BoNTs are synthesized as a single polypeptide chain (150 kDa), which is post-translationally cleaved into a di-chain molecule composed of light chain (LC, 50 kDa) and heavy chain (HC, 100 kDa). LC is the catalytic domain and a zinc-endopeptidase, while HC is further divided into two sub-domains of equal molecular mass called the translocation domain (Hn) and the membrane binding domain (Hc). Inhibition of neurotransmission takes place by proteolysis of one of the SNARE proteins that mediate cell secretion. Synaptobrevin (or VAMP) was identified as the BoNT/D specific substrate and is cleaved at the Lys59-Leu60 position.

The crystal of LHn/D diffracted at 2.3 Å resolution in space group P6422 with cell dimensions a = b = 173, c = 222 Å; α = β = 90, γ = 120°. Despite the large unit cell, a single molecule was present in the asymmetric unit corresponding to an unusually high solvent content of 75%. The X-ray crystal structure presents the two domains, LC and Hn, in a close interaction. No electron density was observed for regions 442–457 (between the two domains), residues 494–510, and the C-terminal poly-histidine tag (last fifteen residues), all in solvent-accessible areas. Additionally, one of the most intriguing features of BoNT, the ‘belt’ region (residues 458–547), which is part of Hn and surrounds LC, was visible in the electron density map (despite high solvent content in the crystal) in the structure presented here and highlights the intricate interactions between the two domains. A PISA22 analysis shows that the LC-belt interaction is supported by over 40 potential hydrogen bonds and 2 salt bridges, making up a 3373 Å2 contact area. Loss of the zinc ion was confirmed with a local rearrangement of the active site residues. Mutation of the zinc-coordinating H233 to tyrosine caused displacement of the catalytic ion, replaced in its position with the Y233 hydroxyl group. Overall, the role of the zinc ion appears mostly catalytic with little impact on the structural integrity of the light chain.

> MTWPVKDFNYSDPVNDNDILYLRIPQNKLITTPVKAFMITQNIWVIPERFSSDTNPSLSKPPRPTSKYQSYYDPSYLSTDEQKDTFLKGIIKLFKRINERDIGKKLINYLVVGSPFMGDSSTPEDTFDFTRHTTNIAVEKFENGSWKVTNIITPSVLIFGPLPNILDYTASLTLQGQQSNPSFEGFGTLSILKVAPEFLLTFSDVTSNQSSAVLGKSIFCMDPVIALMHQLTYSLHQLYGINIPSDKRIRPQVSEGFFSQDGPNVQFEELYTFGGLDVEIIPQIERSQLREKALGHYKDIAKRLNNINKTIPSSWISNIDKYKKIFSEKYNFDKDNTGNFVVNIDKFNSLYSDLTNVMSEVVYSSQYNVKNRTHYFSRHYLPVFANILDDNIYTIRDGFNLTNKGFNIENSGQNIERNPALQKLSSESVVDLFTKVCVDKSEEKLYDDDDKDRWGSSLQCIKVKNNRLPYVADKDSISQEIFENKIITDETNVQNYSDKFSLDESILDGQVPINPEIVDPLLPNVNMEPLNLPGEEIVFYDDITKYVDYLNSYYYLESQKLSNNVENITLTTSVEEALGYSNKIYTFLPSLAEKVNKGVQAGLFLNWANEVVEDFTTNIMKKDTLDKISDVSVIIPYIGPALNIGNSALRGNFNQAFATAGVAFLLEGFPEFTIPALGVFTFYSSIQEREKIIKTIENCLEQRVKRWKDSYQWMVSNWLSRITTQFNHINYQMYDSLSYQADAIKAKIDLEYKKYSGSDKENIKSQVENLKNSLDVKISEAMNNINKFIRECSVTYLFKNMLPKVIDELNKFDLRTKTELINLIDSHNIILVGEVDRLKAKVNESFENTMPFNIFSYTNNSLLKDIINEYFNLEAHHHHHHHHHH> GSSSLLDPLKIADQSVDLNLKLMKWRILPDLNLDIIKNTK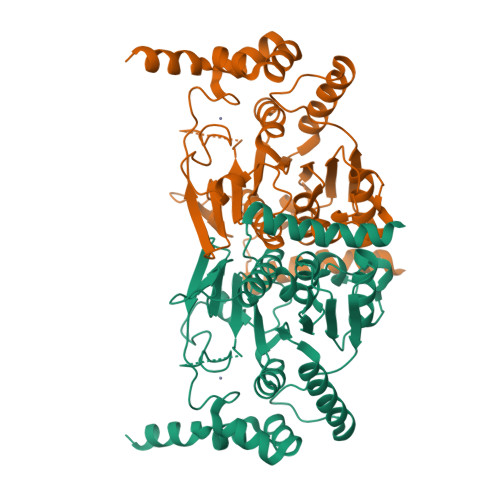VLLLGAGTLGCYVSRALIAWGVRKITFVDNGTVSYSNPVRQALYNFEDCGKPKAELAAASLKRIFPLMDATGVKLSIPMIGHKLVNEEAQHKDFDRLRALIKEHDIIFLLVDSRESRWLPSLLSNIENKTVINAALGFDSYLVMRHGNRDEQSSKQLGCYFCHDVVAPTDSLTDRTLDQMCTVTRPGVAMMASSLAVELMTSLLQTKYSGSETTVLGDIPHQIRGFLHNFSILKLETPAYEHCPACSPKVIEAFTDLGWEFVKKALEHPLYLEEISGLSVIKQEVERLGNDVFEWEDDESDEIA(3~{S})-~{N}-[(3-chloranyl-5-fluoranyl-phenyl)methyl]-3-oxidanyl-2-oxidanylidene-1-(2-oxidanylidene-3,4-dihydro-1~{H}-quinolin-6-yl)pyrrolidine-3-carboxamide 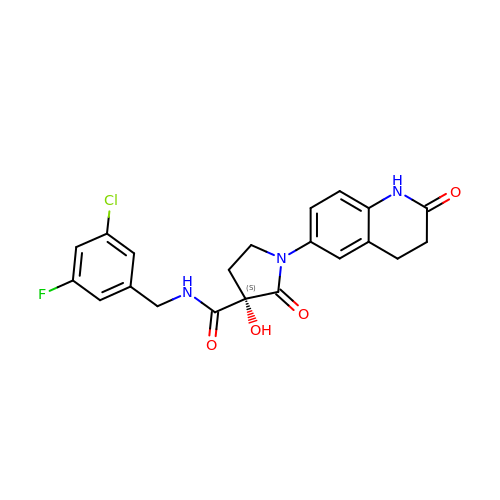| C21 H19 Cl F N3 O4 | RMWSKRBLJAUOOY-NRFANRHFSA-N>[4x]MKHILLITGAGKGIGRAIALEF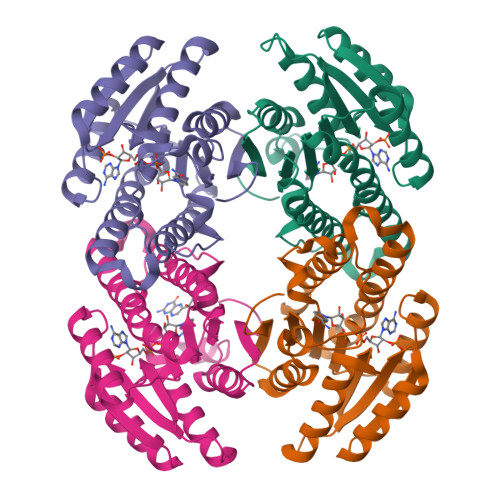ARAARHHPDFEPVLVLSSRTAADLEKISLECRAEGALTDTITADISDMADVRRLTTHIVERYGHIDCLVNNAGVGRFGALSDLTEEDFDYTMNTNLKGTFFLTQALFALMERQHSGHIFFITSVAATKAFRHSSIYCMSKFGQRGLVETMRLYARKCNVRITDVQPGAVYTPMWGKVDDEMQALMMMPEDIAAPVVQAYLQPSRTVVEEIILRPTSGDIQDD>MGSSHHHHHHSSGRENLYFQGVRPAVIAATGLYTPPDSVSNAELVEAFNTYVANFNAANKARIEAGEIEPLQPSSSEFIEKASGIKSRYVVAKPGIVDPDVMRPIIPERSNDELSILAEMAVTAAEQAIERWGKPRERIGAVLCACSNMQRAYPAMAIEVQNALGLGGFAFDMNVACSSATFGLKTAADFVGGGSVDAVLMVNPEICSGHLNFRDRDSHFIFGDVATAAIVERADDAQGGWSILGTKLKTQFSNN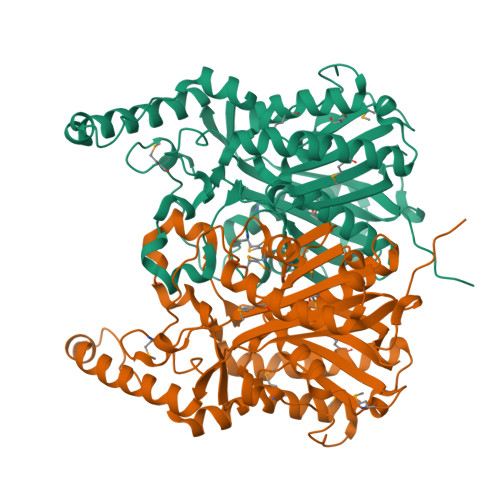IRNNAGFLNRAWPEGRDKADKLFVQQGRKVFKEVVPLVSEMIIEHAREIGIDPHGLKRMWLHQANINMNEIIGRKVLGRDPTRDENVIILDDYANTSSAGSIIAFHKHQDDMAQGDLGLICSFGAGYSAGTVFVQKR[2x]>GVGDLIRKAVSVIKNIV[2x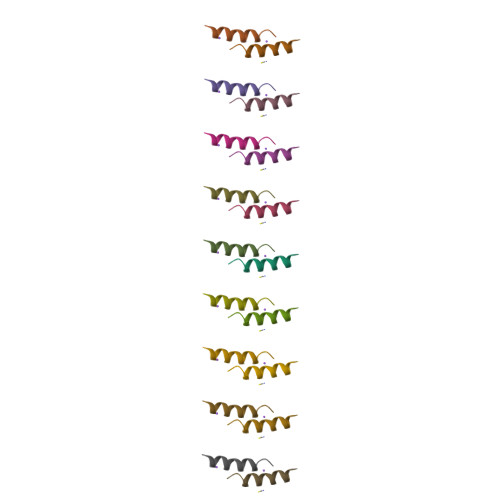]>[2x]PGAVGDGPPRVDFPRSRLRFKEKLGEGQFGEVHLCEVDSPQDLVSLDFPLNVRKGHPLLVAVKILRPDATKNARNDFLKEVKIMSRLKDPNIIRLLGVCVQDDPLCMITDYMENGDLNQ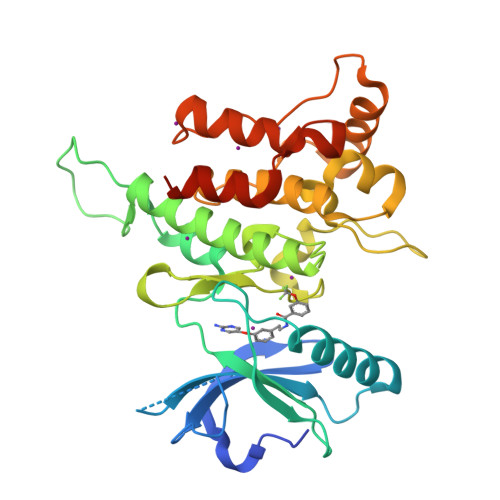FLSAHQLEDKAAEGAPGDPTISYPMLLHVAAQIASGMRYLATLNFVHRDLATRNCLVGENFTIKIADFGMSRNLYAGDYYRVQGRAVLPIRWMAWECILMGKFTTASDVWAFGVTLWEVLMLCRAQPFGQLTDEQVIENAGEFFRDQGRQVYLSRPPACPQGLYELMLRCWSRESEQRPPFSQLHRFLAEDALNTVHHHHHH> IETVPVKLKPGMDGPKVKQWPLTEEKIKALVEICTEMEKEGKISKIGPENPYNTPVFAIKKKDSTKWRKLVDFRELNKRTQDFWEVQLGIPHPAGLKKKKSVTVLDVGDAYFSVPLDEDFRKYTAFTIPSINNETPGIRYQYNVLPQGWKGSPAIFQSSMTKILEPFKKQNPDIVIYQYMDDLYVGSDLEIGQHRTKIEELRQHLLRWGLTTPDKKHQKEPPFLWMGYELHPDKWTVQPIVLPEKDSWTVNDIQKLVGKLNWASQIYPGIKVRQLCKLLRGTKALTEVIPLTEEAELELAENREILKEPVHGVYYD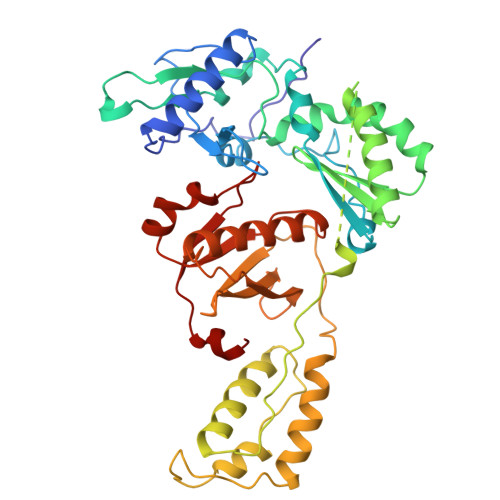PSKDLIAEIQKQGQGQWTYQIYQEPFKNLKTGKYARMRGAHTNDVKQLTEAVQKITTESIVIWGKTPKFKLPIQKETWETWWTEYWQATWIPEWEFVNTPPLVKLWY>FVPEEFWEVDASTTTPSGEALALQVTHQNDKPFRPVNKEQTQAAVSLLEKARYSVLEREDKPTTSKPGAPFITSTLQQAASTRLGFGVKKTMMMAQRLYEAGYITYMRTDSTNLSQDAVNMVRGYISDNFGKKYLPESPNQYASKENSQEAHEAIRPSDVNVMAESLKDMEADAQKLYQLIWRQFVACQMTPAKYDSTTLTVGAGDFRLKARGRILRFDGWTKVMPALRKGDEDRILPAVNKGDALTLVELTPAQHFTKPPARF[2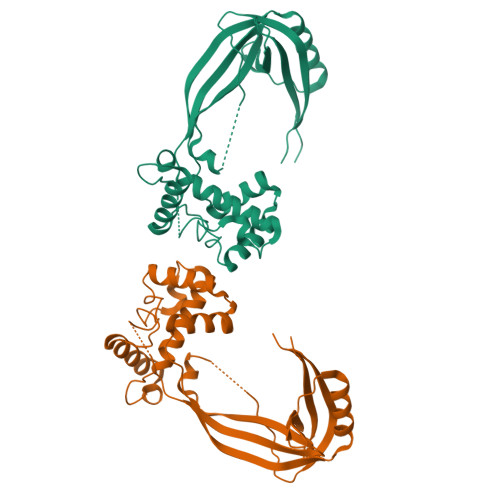x]>[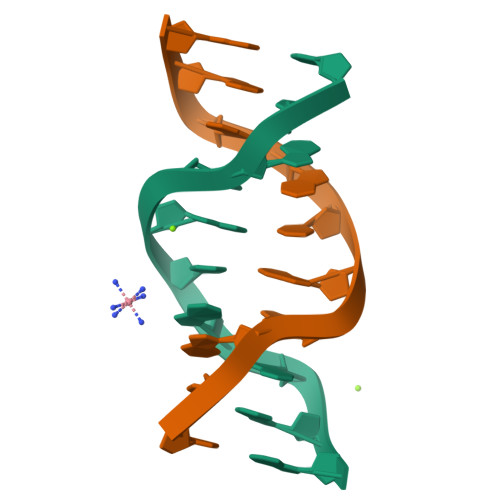2x]CCGAATGAGG> MKSEPLSYLGKDGGPWEIFTEQVDRVVPYLGRLAPLAESLKRPKRVLIVDVPVRLDDGSVAYFEGYRVHHNTARGPAKGGVRYHPEVTLSEVMALAGWMTIKNAAVGLPYGGGKGGIRVDPRKLSPGELERLTRRYTSEIGILLGPDRDIPAPDVNTGEREMAWMMDTYS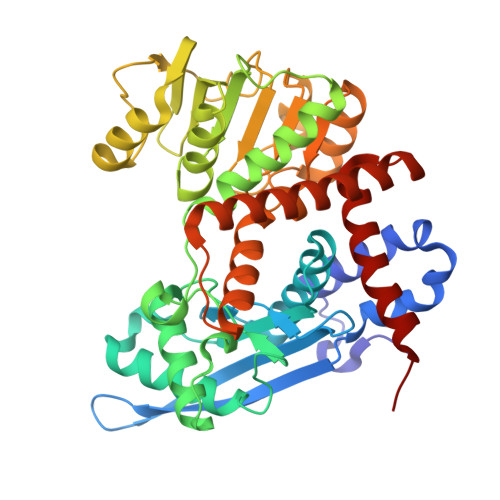MNVGRTVPGVVTGKPIALGGSLGRRDATGRGVFITAAAAAEKIGLQVEGARVAIQGFGNVGNAAARAFHDHGARVVAVQDHTGTVYNEAGIDPYDLLRHVQEFGGVRGYPKAEPLPAADFWGLPVEFLVPAALEKQITEQNAWRIRARIVAEGANGPTTPAADDILLEKGVLVVPDVIANAGGVTVSYFEWVQDFNSYFWTEEEINARLERVLRNAFEAVWQVAQEKKIPLRTAAYVVAATRVLEARALRGLYP FtsZ is a tubulin homolog GTPase protein that is widely conserved in bacteria and plays a key role in a complex called divisome, which carries out cell division. FtsZ polymerizes into protofilaments to form the Z-ring that acts as a scaffold for accessory proteins during cell division. FtsZ treadmilling, a motion in which the protofilament polymerizes in one end (plus-end) and depolymerizes in the other end (minus-end), drives cell wall synthesis that constricts the Z-ring to form a septum of the cell. In order to aid high-resolution structure determination of the FtsZ protofilament, we developed a monobody (Mb) that binds to both KpFtsZ and EcFtsZ with high affinity.

We determined the solution structure of a single straight protofilament of KpFtsZ by cryoEM, in which KpFtsZ was in the T conformation with GMPCPP bound. We prepared cryoEM specimen grids for the thin filaments with 0.5 mg ml–1 KpFtsZ supplemented with 1 mM GMPCPP. After refining the helical parameters, the reconstituted 3D map represented a single protofilament of KpFtsZ with a helical rise of 44.02 Å and a helical twist of 0.025°. Although the resolution of the final reconstructed 3D map reached 3.03 Å, the quality of the map was not enough to trace the main chain in some regions and to visualize many side chains, and the resolution estimated from the atomic model (dmodel) was limited to 3.5 Å. However, the map enabled us to identify the β-sheet in the C-terminal domain (CTD) and the H7 helix and to confirm that KpFtsZ adopted the T conformation. GMPCPP was present in the nucleotide-binding pocket where a clear density of γ-phosphate was observed, but the density was not clear enough to determine the accurate position and conformation of the GMPCPP. The density corresponding to the T7 loop, which contributes to GTP hydrolysis, was also not resolved well but bound a metal ion. The main chain carbonyls of Leu199, Arg202, Val208 and the side chain of Asn207 were coordinated to the metal ion, as is often seen in the T conformation crystal structures. KpFtsZ in the cryoEM structure of the single protofilament was, however, clearly distinct from the other three and adopted the T conformation (r.m.s.d. = 1.887 Å over 280 Cα atoms for the P21 dataset, 1.935 Å over 279 Cα atoms for the P212121 dataset, and 1.858 Å over 276 Cα atoms for the double-helical tube dataset). The KpFtsZ monomer in the single protofilament showed the typical feature of the T conformation: the central H7 helix shifted downwards, and the CTD rotated outwards to open the inhibitor-binding pocket. The T conformation protofilament in the single protofilament structure was stabilized by larger interface areas (1114 Å2) and lower free energy (ΔG = –17.8 kcal mol–1).

>[4x]GHMFEPMELTNDAVIKVIGVGGGGGNAVEHMVRERIEGVEFFAVNTDAQALRKTAVGQTIQIGSGITKGLGAGANPEVGRNAADEDREALRAALDGADMVFIAAGMGGGTGTGAAPVVAEVAKDLGILTVAVVTKPFNFEGKKRMAFAEQGITELSKHVDSLITIPNDKLLKVLGRGISLLDAFGAANDVLKGAVQGIAELITRPGLMNVDFADVRTVMSEMGYAMMGSGVASGEDRAEEAAEMAISSPLLEDIDLSGARGVLVNITAGFDLRLDEFETVGNTIRAFASDNATVVIGTSLDPDMNDELRVTVVATGIGMDKRPEITLVTNKQVQQPVMDRYQQHGMSPLTQEQKPAAKVVNDNTPQTAKEPDYLDIPAFLRKQAD>[2x]MVMNPERSLSDFMRSSQERVERALDARLPAADRMPERLHQAMRYSVLGGGKRMRPLLTYATGQTIGVAADLLDGPACAVEFIHVYSLIHDDLPAMDDDDLRRGKPTCHKAYDEATAILAGDGLQALAFHVLAQDPSIAVPAENRIAMIETLAKASGPAGMVGGQAIDLASVGKKLDLPGLENMHIRKTGALIRASVRLACLARPGLPAEQFDRL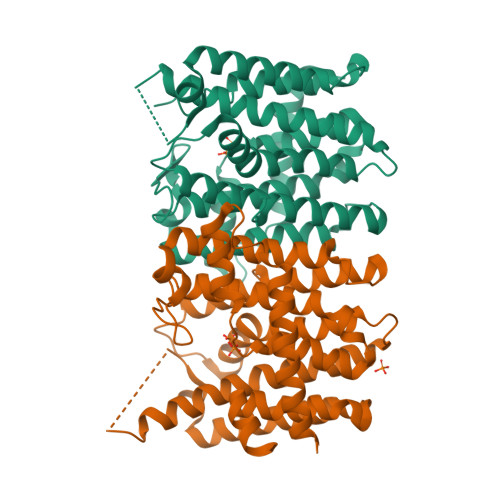DHYAKCIGLAFQIQDDILDEESDTQTLGKTRGKDRDHNKPNYPALLGLSGAKEKAEEMHEAALESLAGFGPEADLLRELARFIIQRQSAENLYFQSHHHHHHWSHPQFEK> AVRQRVIPVYQVNNLEEICQLIIQAFEAGVDFQESADSFLLMLCLHHAYQGDYKLFLESGAVKYLEGHGFRFEVKKRDGVKRLEELLPAVSSGKNIKRTLAAMPEEETTEANAGQFLSFASLFLPKL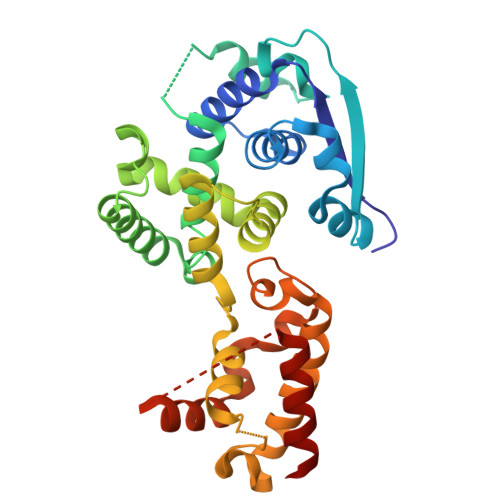VVGEKACLEKVQRQIQVHAEQGLIQYPTAWQSVGHMMVIFRLMRTNFLIKFLLIHQGMHMVAGHDANDAVISNSVAQARFSGLLIVKTVLDHILQKTERGVRLHPLARTAKVKNEVNSFKAALSSLAKHGEYAPFARLLNLSGVNNLEHGLFPQLSAIALGVATAHGSTLAGVNVGEQYQQLREAATEAE> MSNFINIHVLISHSPSCLNRDDMNMQKDAIFGGKRRVRISSQSLKRAMRKSGYYAQNIGESSLRTIHLAQLRDVLRQKLGERFDQKIIDKTLALLSGKSVDEAEKISADAVTPWVVGEIAWFCEQVAKAEADNLDDKKLLKVLKEDIAAIRVNLQQGVDIALSGRMATSGMMTELGKVDGAMSIAHAITTHQVDSDIDWFTAVDDLQEQGSAHLGTQEFSSGVFYRYANINLAQLQENLGGASREQALEIATHVVHMLAT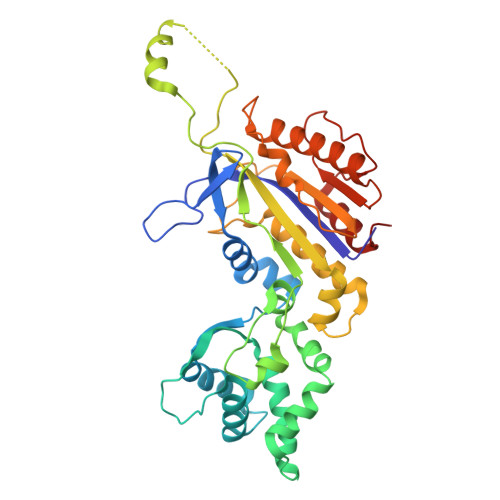EVPGAKQRTYAAFNPADMVMVNFSDMPLSMANAFEKAVKAKDGFLQPSIQAFNQYWDRVANGYGLNGAAAQFSLSDVDPITAQVKQMPTLEQLKSWVRNNGEA> CTANEQAGKEGSHDKAKTSGEKVLYVNNENEPTSFDPPIGFNNVSWQPLNNIMEGLTRLGKDHEPEPAMAEKWSVSKDNKTYTFTIRENAKWTNGDPVTAGDFEYAWKRMLDPKKGASSAFLGYFIEGGEAYNSGKGKKDDVKVTAKDDRTLEVTLEAPQKYFLSVVSNPAYFPVNEKVDKDNPKWFAESDTFVGNGPFKLTEWKHDDSITMEKSDTYWDKDTVKLDKVKWAMVSDRNTDYQMFQSGELDTAYVPAELSDQLLDQDNVNIVDQAGLYFYRFNVNMEPFQNENIRKAFAMAVDQEEIVKYVTKNNEKPAHAFVSPGFTQPDGKDFREAGGDLIKPNESKAKQLLEKGMKEENYNKLPAITLTYSTKPEHKKIAEAIQQKLKNSLGVDVKLANMEWNVFLEDQKALKFQFSQSSFLPDYADPISFLEAFQTGNS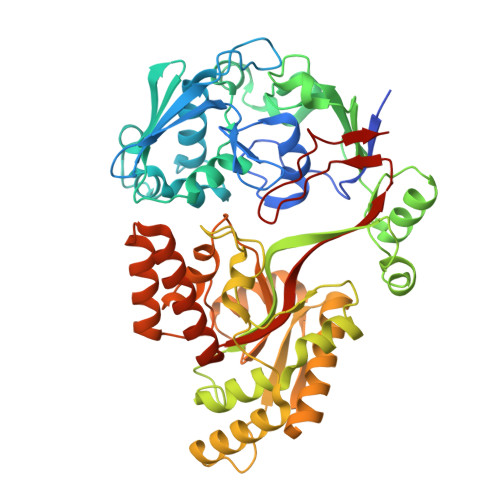MNRTGWANKEYDQLIKQAKNEADEKTRFSLMHQAEELLINEAPIIPVYFYNQVHLQNEQVKGIVRHPVGYIDLKWADKN> MRRFCTARVSSYVKRAPLLLPRGGRRWRSGAGTTADGGGEKEYIADSFESTAGSNAYAAMELAAEARREIHELWLSAETALEREKRVQQVAALIEKYKLDPSTPREADVSRGLGDAFDRLLLLCLPLGKTDAKGTDNLERLMHLAGRNGREL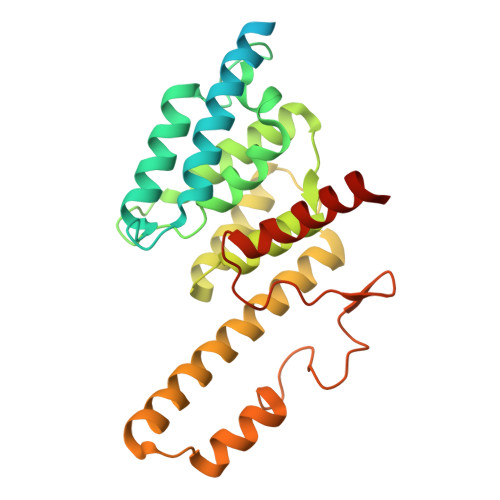SVRTIQHLFARTDSFAEALAVFYTMRRCHVAMNMEAYYSMLYSLQRLEEEGWGQHFRNEYEENGAPSEQAMDFIVKGISNALLPENKPWLGRVMFQDRNVPDRRYDTRDFDELDTAWTQRYKSGTPAGAH>[2x]GNEEIPGLEVEEIDNGVFLHKSYSRVEGWGLVSSNGLVV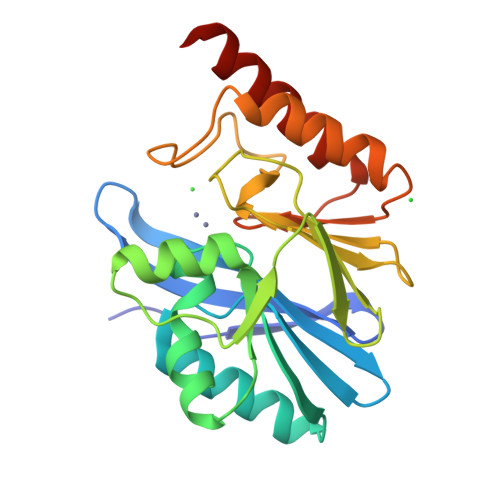ISGGKAFIIDTPWSESDTEKLVDWIRSKKYELAGSISTHSHEDKTAGIKWLNGKSITTYASALTNEILKREGKEQARSSFKGNEFSLMDGFLEVYYPGGGHTIDNLVVWIPSSKILYGGCFIRSLESSGLGYTGEAKIDQWPQSARNTISKYPEAKIVVPGHGKIGDFELLKHTKVLAEKASNKANHGDR L-LYSYL-N~5~-[(Z)-(2,2-DIHYDROXYHYDRAZINO)(IMINO)METHYL]-L-ORNITHINAMIDE 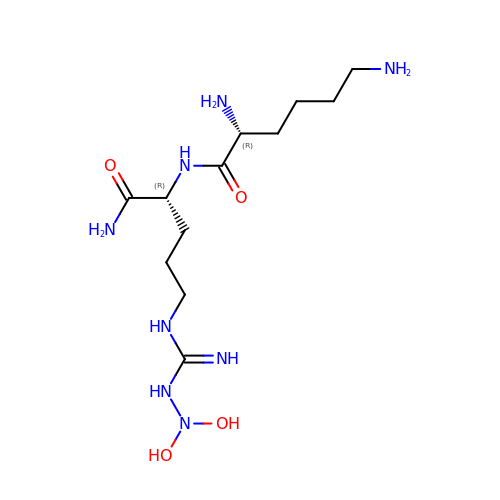| C12 H28 N8 O4 | VKBOUZQMRKGFCB-RKDXNWHRSA-N> MTTAVARLQPSASGAKTRPVFPFSAIVGQEDMKLALLLTAVDPGIGGVLVFGDRGTGKSTAVRALAALLPEIEAVEGCPVSSPNVEMIPDWATVLSTNVIRKPTPVVDLPLGVSEDRVVGALDIERAISKGEKAFEPGLLARANRGYLYIDECNLLEDHIVDLLLDVAQSGEN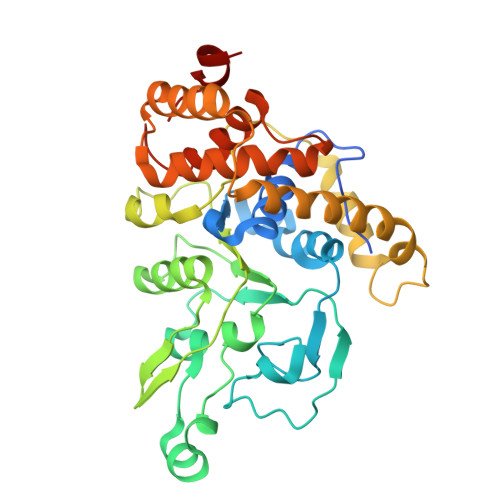VVERDGLSIRHPARFVLVGSGNPEEGDLRPQLLDRFGLSVEVLSPRDVETRVEVIRRRDTYDADPKAFLEEWRPKDMDIRNQILEARERLPKVEAPNTALYDCAALCIALGSDGLRGELTLLRSARALAALEGATAVGRDHLKRVATMALSHRLRRDPLDEAGSTARVARTVEETLP>MFNR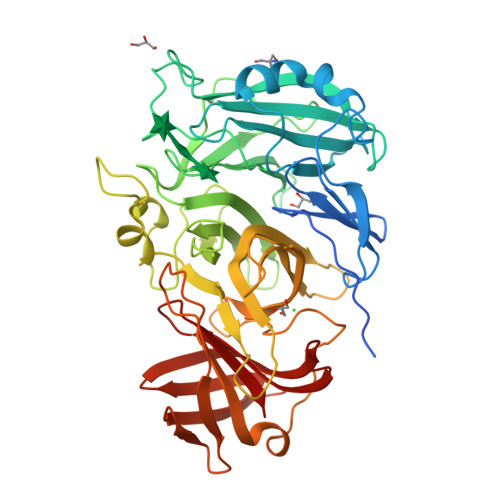LFRVCFLAALIMAFTLPNSVYAQKPIFKEVSVHDPSIIETNGTFYVFGSHLASAKSNDLMQWQQLTTSVSNDNPLIPNVYEELKETFEWAQSDTLWAADVTQLADGKYYMYYNACRGDSPRSAMGVAVADNIEGPYKNKGIFLKSGMEGTSSDGTPYDATKHPNVVAPHTFFDKDGKLWMVYGSYSGGIFILEMNPKTGFPLPGQGYGKKLLGGNHSRIEGPYVLYNPDTQYYYLYLSYGGLDATGGYNIRVARSKKPDGPYYDAEGNPMLDVRGKGGTFFDDRSIEPYGVKLMGSYTFETENEKGTGYVSPGHNSAYYDEKTGRSYLIFHTRFPGRGEEHEVRVHQLFMNKDGWPVAAPYRYAGETLKEVKQKDITGTYKLIQHGKDISADIKQTINIQLNKNHTISGEMTGTWRKTGKNTADITLAGKKYNGVFLRQWDSVREKNVMTFSVLNTSGEAVWGSKL[2x]> DCPSDWSSYEGHCYKPFSEP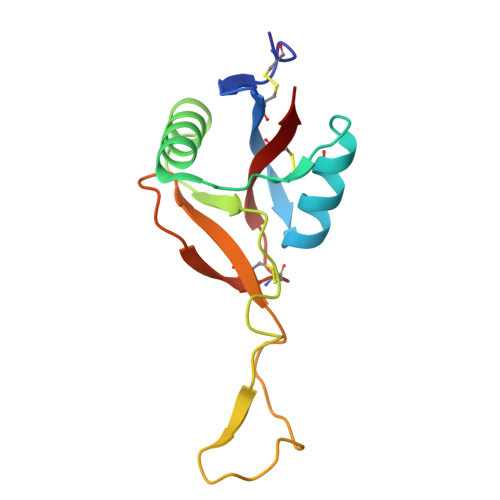KNWADAENFCTQQHAGGHLVSFQSSEEADFVVKLAFQTFGHSIFWMGLSNVWNQCNWQWSNAAMLRYKAWAEESYCVYFKSTNNKWRSRACRMMAQFVCEFQA>EVIASGRLEKCVVDGVTEELDCQEKVVVTLTVGNGQSLQTEALEFSLSCLNSPDGRCPCSCSAADPTCACRDLAAPLRVSLTKSPLWASYPLQYLSSFNWKPLEVILRPSNKVCKDGDWEDSPTCGWFSQGGVRVADSQGFCCECSSSQVWDDTFGSSKERTRANLDCDFWSDPLDILIGRKPVSAHCLTFDPQWYSGYELGAASLQFEIAITVEVPTAPSPTTATTSATPRTNNSSSANSTNSTNSPAPQFLSPPAPSTREVLHLGPSVPLASSASRLLSAKLLGDLAMYTQLPAISNQVLMVPQPPAAAAATGSPLDALATNRS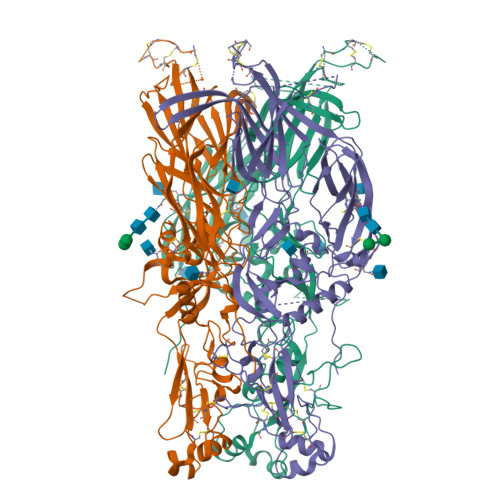AWMLLDKTMLSMDGLACDKVGTGFSAFRYQPSGCGRAPQACLSGQLKDLWEADLARIADGRVPLYMITRFTGGSDTTLQSFSGGPLSFALPVTSHSQSLVTLSVAADGVRLVTNRSPGKITGAAVCRFAGTSCGGFEAVAARGYIYVNITNTGRLDSDYTLTVSNCSSNVRPIEARTLAVRAGSAASLDPPMELYVEDQAAAAARTCTVSLYDSVGAVTDSLTLSFYTNATQLHHHHHH[3x]> GSHMSSAF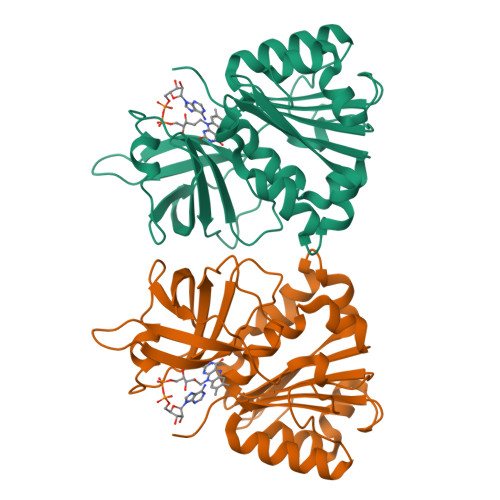GAETVLEVRHWTDAYFSFTTTRDAGFRFENGQFVMIGLETETRPLLRAYSIASANWEEHLEFFSIKVPDGPLTSRLQHIQPGDKVLVGKKPTGTLLISDLHPGRNLYLLGTGTGLAPWLSIIKDPETYERFDKVILTQGVRFVQDLAYRDYFERELPQHEFLGDLLREKLLYYPAVTRETFANQGRLTELMADGRMQQTLGLPTLDPANDRFMICGSPQMLADLRSLLDSRGFQTSPRIGTPGHYVFERAFVEK>MKHHHHHHPMASAATESATATATLEETLAQRLRLGSLEPDGLSYKESFIVRSYEVGVNKTATVETIANLLQEVGCNHAQSVGFSTDGFATTTTMRLLRLIWVTARMHIEIYKYPAWGDV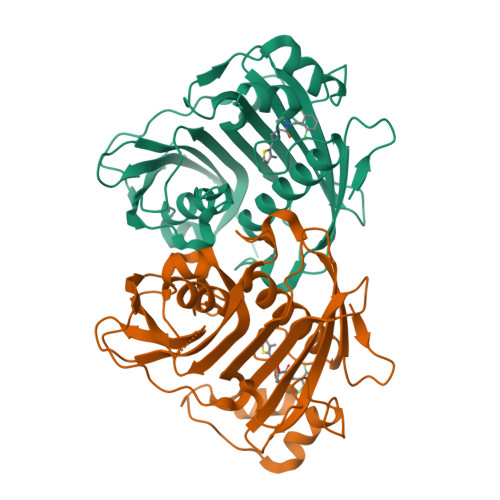VEIETWCQEDGKIGTRRDWIIKDYSTGVVIGRATSKWVMMNQDTRRLQRVNDEVREEYLIFCPRTPRLAFPEEDSDSLKKIPKLEEPAQSSKLGLVPRRADLDMNQHVNNVTYIGWVLESIPQEIIDTHELQTITLDYRRECQHDDIVDSLSSREFGDTPQNGNHSTGRKEGECQFLHFLKLSGSGLEINRGRTQWRRLAK[4x]>MLLQASQATQSVWKTLNKWLPPLSRDKDWWWKTLGPQINTLLTEADYDLNERYEALLLLYRWVVPEMGPRPRSSVAPSKSFMTDDHSPIEYSWKWISGNKKPEIRYAVELVSPLAGSKQDPFNQIPTRNLVYNLAKIIPELDLTWFEHFWHELLGPGSPTTSTSGVLTKGSTVFAALEMLHGHLSVKVYFIPVETPDFSAWHQIKHAIEASGCPNLEALNHVDAYLSSHDDGRQLRPFMLAIDLVEPAASRLKIYARSNQTSFRFVRDVMTIGGLRTDLDRSIEKFSDLWKRALGLDPDTPPEDELPKVDHLTSGAVFNFDVAPKSQIPEVKAYIPVRHYANNDLQAALGLIGYLEDHGHGGYSQSYLRGLDMLAPSGQLDQATGV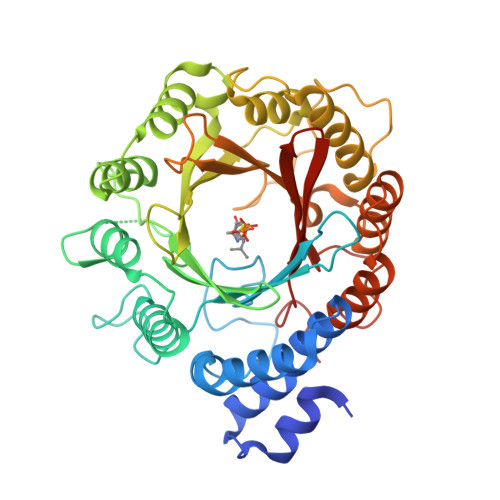QTYFAVACQGEDLSLTSYLNPQFYAAFQEPERT[4x]> NDPGKMLKDAIDKQVAGALVAGTTTSTHSVATDSTPALQAAETGATSTARDESMIETRTIVPTHGIHETSVESFFGRSSLVGMPLLATGTSITHWRIDFREFVQLRAKMSWFTYMRFDVEFTIIATSSTGQNVTTEQHTTYQVMYVPPGAPVPSNQDSFQWQSGCNPSVFADTDGPPAQFSVPFMSSANAYSTVYDGYARFMDTDPDRYGILPSNFLGFMYFRTLEDAAHQVRFRIYAKIKHTSCWIPRAPRQAPYKKRYNLVFSGDSDRICSNRASLTSY;> SPSAEACGYSDRVAQLTLGNSTITTQEAANICVAYGCWPAKLSDTDATSVDKPTEPGVSADRFYTLRSKPWQADSKGWYWKLPDALNNTGMFGQNAQFHYIYRGGWAVHVQCNATKFHQGTLLVLAIPEHQIATQEQPAFDRTMPGSEGGTFQEPFWLEDGTSLGNSLIYPHQWINLRTNNSATLILPYVNAIPMDSAIRHSNWTLAIIPVAPLKYAAETTPLVPITVTIAPMETEYNGLRRAIASNQ;> GLPTKPGPGSYQFMTTDEDCSPCILPDFQPTPEIFIPGKVNNLLEIAQVESILEANNREGVEGVERYVIPVSVQDALDAQIYALRLELGGSGPLSSSLLGTLAKHYTQWSGSVEITCMFTGTFMTTGKVLLAYTPPGGDMPRNREEAMLGTHVIWDFGLQSSITLVIPWISASHFRGVSNDDVLNYQYYAAGHVTIWYQTNMVIPPGFPNTAGIIMMIAAQPNFSFRIQKDREDMTQTAILQ;> GAQGGSTINYNNINYYSHAASAAQNKQDFTQDPSKFTQPIADVIKETAVPLK

Enterovirus-E (EV-E), formerly known as bovine enterovirus, a surrogate for poliovirus (PV), belongs to one of the best studied genera, the enteroviruses, which include PV and the human rhinoviruses. Picornaviruses assemble to form icosahedral particles with pseudo T = 3 symmetry, enclosing a single copy of the genome, gRNA, ~7-10k nts long. The polyprotein is processed by a virally-encoded protease into VP0, VP3 and VP1. VPs 1–3 form the outer surface of the viral capsid with VP1 located around the five-fold axes, and VP2 and VP3 alternating around two- and three-fold axes.

The structure of the EV-E virion was determined by cryo-EM single particle analysis at 2.2 Å resolution. Atomic models of the four capsid proteins reveal typical picornavirus-like folds, having jelly-roll motifs with extended N-terminal arms that are not all complete within the map. The cryo-EM density allows us to build atomic models for more of these features than was possible in the previous X-ray map. The atomic coordinates for VP1, VP2 and VP4 were updated from the X-ray structure and ~20% of the previously missing residues were unequivocally assigned (regions in pink). The VP1 N-terminal domain was updated with 10 additional residues, which extend to the innermost surface of the five-fold pores. The structure in this region was corrected and modelled according to the EM density map, which is similar to that of the recently determined EV-F X-ray structure. This density map also allowed us to assign the VP2 sequence up to residue Y9, which is located precisely at the three-fold axis. VP4 was assigned up to residue G21 (orientated towards the five-fold axis) and its C-terminus completed up to K69. There are two myristic acid groups associated with the structure. One is bound as the VP1 pocket factor. A second myristate is visible at the end of a disconnected portion of protein density, which we assigned to the G2-Q4 position of VP4 both because of its location with respect to the remainder of VP4 and the known myristylation site at the N-terminus of poliovirus VP4.> PISPIETVPVKLKPGMDGPKVKQWPLTEEKIKALVEICTEMEKEGKISKIGPENPYNTPVFAIKKKDSTKWRKLVDFRELNKRTQDFWEVQLGIPHPAGIKKKKSVTVLDVGDAYFSVPLDEDFRKYTAFTIPSINNETPGIRYQYNVLPQGWKGSPAIFQSSMTKILEPFRKQNPDIVIYQYMDDLYVGSDLEIGQHRTKIEELRQHLLRWGLTTPDKKHQKEPPFLWMGYELHPDKWTVQPIVLPEKDSWTVNDIQKLVGKLNWASQIYPGIKVRQLCKLLRGTKALTEVIPLTEEAELELAENREILKEPVHGVYYDPSKDLIAEIQKQGQGQWTYQIYQEPFKNLKTGKYARMRGAHTNDVKQLTEAVQKITTE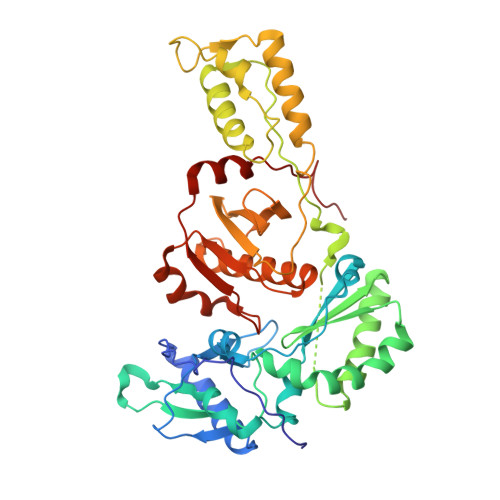SIVIWGKTPKFKLPIQKETWETWWTEYWQATWIPEWEFVNTPPLVKLWYQLEKEPIVGAETF> QIGWRREGIKYRRNELFLDVLESVNLLMSPQGQVLSAHVSGRVVMKSYLSGMPECKFGMNDKIVIEKQGKGTADETSKSGKQSIAIDDCTFHQCVRLSKFDSERSISFIPPDGEFELMRYRTTKDIILP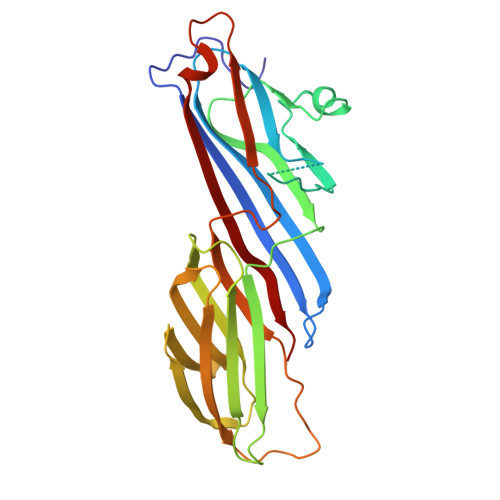FRVIPLVREVGRTKLEVKVVIKSNFKPSLLAQKIEVRIPTPLNTSGVQVICMKGKAKYKASENAIVWKIKRMAGMKESQISAEIELLPTNDKKKWARPPISMNFEVPFAPSGLKVRYLKVFEPKLNYSDHDVIKWVRYIGRSGIYETRC> MASPENPWLWAVLVLLLALSAFFSASETAITTLYPWKLKELAESKNGPFRLLAEDITRFLTTILVGNNLVNIAATALATELATQAFGSAGVGVATGAMTFLILFFGEITPKSLAVHHAEAIARLAAWPIYGLSVLFYPV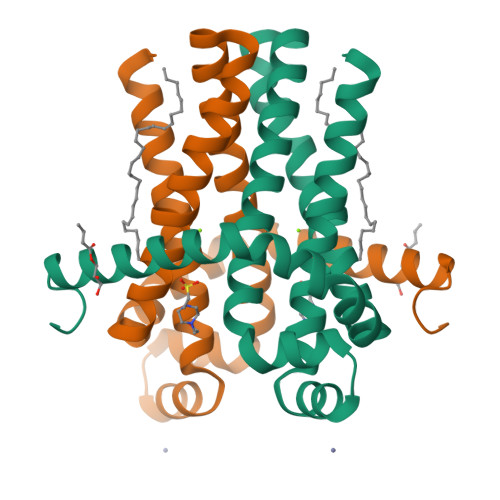GRFFSLVSGGLLRLLGLEPRLESSGLEVLFQ>[4x]MAHTGRMFKIEAAEIVVARLPLKFRFETSFGVQTHKVVPLLILHGEGVQGVAEGTMEARPMYREETIAGALDLLRGTFLPAILGQTFANPEAVSDALGSYRGNRMARAMVEMAAWDLWARTLGVPLGTLLGGHKEQVEVGVSLGIQADEQATVDLVRRHVEQGYRRIKLKIKPGWDVQPVRATREAFPDIRLTVDANSAYTLADAGRLRQLDEYDLTYIEQPLAWDDLVDHAEL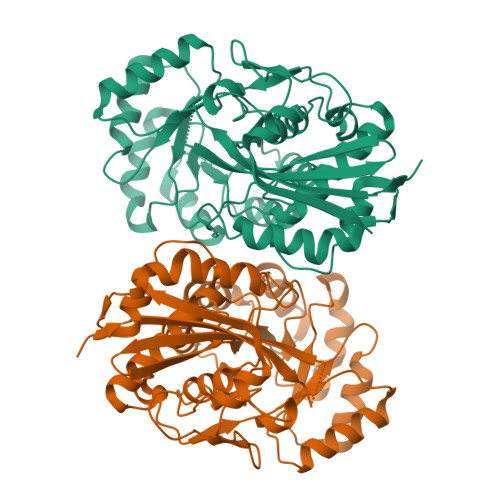ARRIRTPLCLDESVASASDARKALALGAGGVINLKVARVGGHAESRRVHDVAQSFGAPVWCGGMLESGIGRAHNIHLSTLSNFRLPGDTSSASRYWERDLIQEPLEAVDGLMPVPQGPGTGVTLDREFLATVTEAQEEHRA Among type II receptors, TGFβR2 and AMHR2 only interact functionally with a select number of GFs, whereas ACVR2A, ACVR2B, and BMPR2 are promiscuous and can form signaling and nonsignaling complexes with an overlapping group of over 30 GFs, including homodimeric and heterodimeric activins, inhibins, bone morphogenetic proteins (BMPs), growth and differentiation factors (GDFs), Nodal, and Lefty. At the most basic level, TGF-β pathways are activated when a dimeric GF forms a signaling complex with both receptor types, triggering a phosphorylation cascade from receptors to R-SMADs that results in R-SMAD–mediated transcriptional responses. Structural and biochemical studies have revealed that the GF-binding domain (GBD) of both type I and type II receptors adopt a similar, “three-finger toxin fold”, where the “fingers” refer to three pairs of antiparallel β-strands that form an extended β-sheet. We have solved the crystal structures of the type II BMPR2 GBD in complex with activin B and of the type II activin Receptor ACVR2A in complex with activin A. We show that BMPR2 and activin type II receptors interact with GFs using a nearly identical mode of binding.

To determine how BMPR2 and its GBD variants interact with GFs, we solved the crystal structure of BMPR2-GBD in complex with activin B, a GF that can bind BMPR2 (28, 35) and that signals via BMPR2 in some cell types. We solved the BMPR2 complex by placing the activin B protomer structure predicted by AlphaFold first. The asymmetric unit of the BMPR2 complex comprised three receptor and three GF protomers, where all biological dimers were related by crystallographic symmetry. BMPR2 binds activin B at its “knuckle epitope”, a convex surface on the GF that is formed by a set of antiparallel β-strands or “fingers”. BMPR2 adopts the three-finger toxin fold seen in other TGF-β family receptors with minor variations in β-strand length, flexibility, and orientation. Its GF-binding interface is similar to that of ACVR2A and consists of a concave surface that harbors a hydrophobic hot spot containing three conserved aromatic residues, Y67, W85, and F115, at its center. By contrast, BMPR2 exhibited significant variability in loop regions and in areas that were not directly involved contacting the GF, possibly reflecting the intermediate-binding affinity of BMPR2 for activin B and the conformational plasticity of the GF-free BMPR2 structures. In fact, loop conformations in the GF-free structure would preclude GF binding, supporting the idea that these loops adopt distinct conformations in the GF-free and GF-bound forms. We also observed a second, substantial interface, which results in the formation of a GF hexamer. Notably, type I receptors interact with the wrist helix at the GF dimer interface and this feature is occluded in the hexameric activin B complex.

>GLECDGRTNLCCRQQFFIDFRLIGWNDWIIAPTGYYGNYCEGSCPAYLAGVPGSASSFHTAVVNQYRMRGLNPGTVNSCCIPTKLSTMSMLYFDDEYNIVKRDVPNMIVEECGCA[3x];>[3x]SQNQERLCAFKDPYQQDLGIGESRISHENGTILCSKGSTCYGLWEKSKGDINLVKQGCWSHIGDPQECHYEECVVTTTPPSIQNGTYRFCCCSTDLCNVNFTENFPPPDTT>MDDKELIEYFKSQMKEDPDMASAVAAIRTLLEFLKRDKGETIQGLRANLTSAIETLCGVDSSVAVSSGGELFLRFISLASLEYSDYSKCKKIMIERGELFLRRISLSRNKIADLCHTFIKDGATILTHAYSRVVLRVLEAAVAAKKRFSVYVTESQPDLSGKKMAKALCHLNVPVTVVLDAAVGYIMEKADLVIVGAEGVVENGGIINKIGTNQMAVCAKAQNKPFYVVAESFKFVRLFPLNQQDVPDKFKYKADTLKVAQTGQDLKEEHPWVDYTAPSLITLL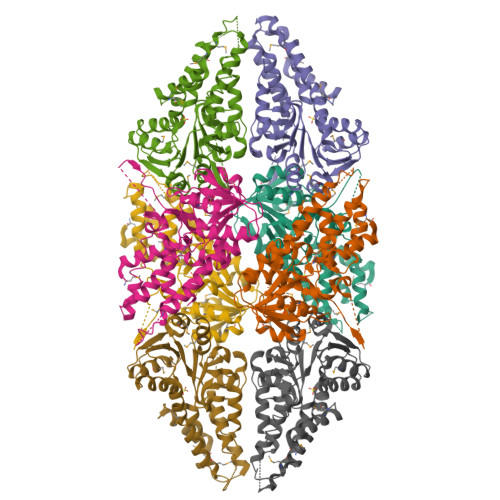FTDLGVLTPSAVSDELIKLYLAAAEHHHHHH[8x]> CG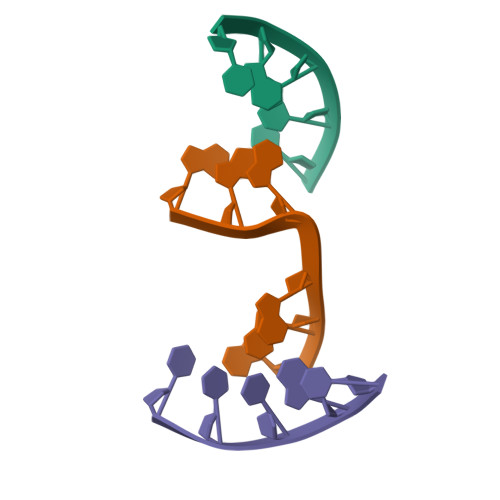CTT;> TTCGC;> AAGGAA>[6x]GSTPAA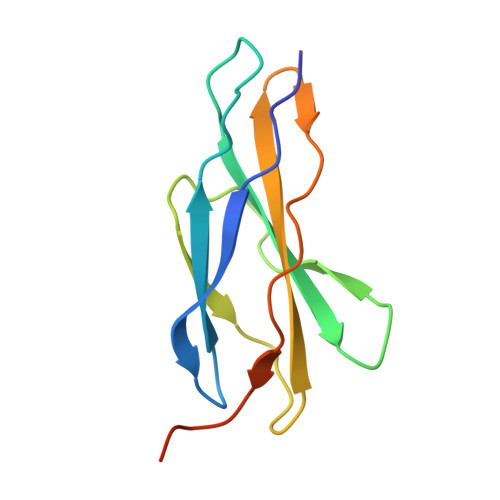PLDVKCLEANKDYIIISWKQPAVDGGSPILGYFIDKCEVGTDSWSQCNDTPVKFARFPVTGLIEGRSYIFRVRAVNKMGIGFPSRVSEPVAALDPAEKARLKSRPS>[2x]XSKIGINGFGRIGRLVLRAALSCGAQVVAVNDPFIALEYMVYMFKYDSTHGVFKGEVKMEDGALVVDGKKITVF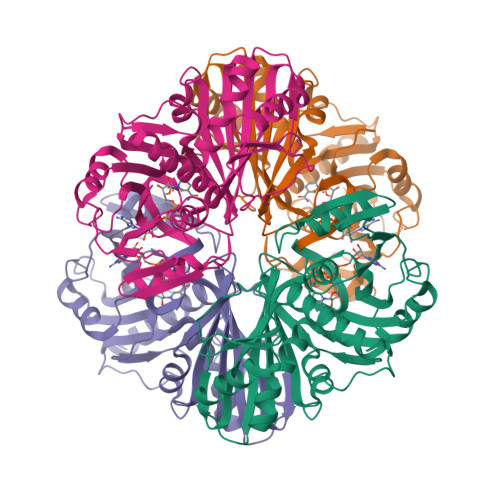NEMKPENIPWSKAGAEYIVESTGVFTTIEKASAHFKGGAKKVVISAPSADAPMFVCGVNLEKYSKDMTVVSNASCTTNCLAPVAKVLHENFEIVEGLMTTVHAVTATQKTVDGPSAKDWRGGRGAAQNIIPSSTGAAKAVGKVIPELDGKLTGMAFRVPTPDVSVVDLTVRLGKECSYDDIKAAMKTASEGPLQGFLGYTEDDVVSSDFIGDNRSSIFDAKAGIQLSKTFVKVVSWYDNEFGYSQRVIDLLKHMQKVDSA>[2x]MADITETQESLPPFRMGEVGSLGLKVRSGRIYEEPRQALRFPESIKTFQLMMRDPSVAASVNIIKMFVRKVNWRFVPPKGKEKDAKMIERANFFNSLMNDMEHDWADFINSVMSFCTYGFCVNEKVYKKRQGKKGKYPSKYNDGLIGWAKLPIRNQTTLDKWYFDSDYRKVIGVRQNLRNVSHTAGAINLGEQPLTRKLPRSKFLLFKYDDEYGNPEGRSPLLNAYVPWKYKVQIEEFEAVGVSRDLVGMPKIGLPPD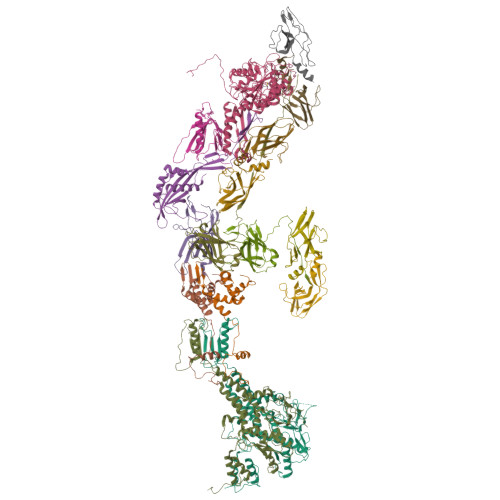YLGEDAEPEKKAFVKYCQEVVNDLIANDRAGLIWPRFIDPETKEDIFEFSLVSRQGAKAYDTGSIIDRYSKQIMMAFMSDVLAMGQSKYGSFSLADSKTSLLAMSVDILLKQIKNVINRDLVAQTYALNMWDDEEHVEIVYDDIETPDIESIGSYVQKTVAVGAMEVDKALSDKLREHIGLEPADESKPVSENLSPNTQSRSGDGYQTAGEGTAKTPSAKDPSTANKANK;>[2x]MCYTGDPANNPLDRVRILCTDTDNNEILIDQSVLEWFYQESGKDEKKAAIKALKYLLFQVAKMGDEKVGGVYLRNSSRFKSLKAVYDDLVKSSVSGLPYAGGINQCDIDMRRQNPCSVKKYTEYGDAVRYYGRDYCERVNGVFIIERDE;> MRLLNRHSFVVKRKVSEDGHYNEDGDWVASQDVVSINCKGNIQPYIKGSVKNGTQIVLPEGIRLTDTRILFTVAELRTSDDVDWTEADIVMIKGHEYEVFMTMDWSEQLAHTSHYEYIIIRRDKMNAVRNSRT;> MQLETAELEKGIVRVLVDVIGHRLARDKNNRPNVIRAYPSDNSNDKGLKPDQPFITVYCQDATTPYGWVLDKFVEDDAVCYRIAFQIPVLITVNGKGAHSIMLELKQRLEMSTTRDYLADMTGASVLDTGAIPNDYTYLNTDFENSAPLVVTLVKNSVLKDERGSIIERVIVDGELVYEEGQEPPEYTIHLDVDSKGVK;> MAMYQQYSPKDVVCSWNGIAIEGFAPDSFLRLQRTSPLVTPVVGAGGQVALTRNADKTGTIEIELMQTSLSNQMLSAIQAKQDDMELEEDISSNFVIYDPSGSVLATGINAWLQELPQIELGRDQNSKTWIFGCEKLDYTSTIPASSV;> MWNPIVNVDITLNTAGTTREGFGLPLFLASTDNFEERIRGYTSLTEVAEDFDESTAAYKAAKQLWSQTPKVTQLYIGRRTMQYTVSIPDTVAEGSEYSLTVAIGGGVSQPFQYTAKENDTALIVLNEFKSQIEASPTIKDGVNASVTGTGASATMIITKAGDNDFVKVTSITPTTSIAATTADTASAALASIETYSTDWYFISAEDRTQQFVLAMASEIQARKKIFFTANADVKALQGTDLTSATDVPAQLAKSKYTRTVCLWHHTAEFDYPEMAYIAYGAPYDAGSIAWGNAQLTGVAASLQPANQRPLISIQKSALDTRSCNFIDLDGGVPVVRRGITSGGEWIDIVRGVDWLESDLKTSLRDLLINQKGGKITYDDTGITRIRQVIETSLQRAVNRKFLSTYTVTVPKASQVALADKKARILKDITFHGILAGAILDVDLKGTVAYE;>[2x]MAEVISISNATRVHSYRGVLIITDELTVEAGSRVSLSGYVSDGGTSDVFTICRLLDAPMNGKQFISNNCNEIVKIPFDSSCLLGVKLYNCENKRVNVNSVEAAFITIDTAFQSPMTVNKESNRLEYIFSQNDYKVLVKGKVYDMIVNVVDESGNHSTILKQKVRFN;>[6x]MGTLTIDGKNKILATLTPTTIVLHNVDPTADPTANKVTQPVAIFFSEPNNGLIASEDTVNITVPASATVSHFSLWDDNSKCVATGALSSPQFFAEEGIYVISSVSIDLNK>MAGKLGKFQMLGFQHWKGLTSDNHLGAIFQQAPQKATNLMVQLLAFYRGKSLDTFLNSFPTREFEDDNEYYWDVIGSSRRNIPLVEARDENGVVVAANAANVGVGTSPFYLVFPEDWFADGEVIVGNLNQVYPFRILGDARMEGTNAVYKVELMGGNTQGVPAERLQQGERFSIEFAPVEKELSRKVGDVRFTSPVSMRNEWTTIRIQHKVAGNKLNKKLAMGIPMVRNLESGKQVKDTANMWMHYVDWEVELQFDEYKNNAMAWGTSNRNLNGEYMNFGKSGNAIKTGAGIFEQTEVANTMYYNTFSLKLLEDALYELSASKLAMDDRLFVIKTGERGAIQFHKEVLKTVSGWTTFVLDNNSTRVVEKVQSRLHSNALSAGFQFVEYKAPNGVRVRLDVDPFYDDPVRNKILHPMGGVAFSYRYDIWYIGTMDQPNIFKCKIKGDNEYRGYQWGIRNPFTGQKGNPYMSFDEDSAVIHRMATLGVCVLDPTRTMSLIPAILQG[30x];>[25x]MVISINQVRQLYVAKALKANTAALTTAGDIVPKADTAKTTLYFQSMSPAGIVASDKINLKHVLYAKATPSEALAHKLVRYSVTLDADVSATPVAGQNYILRLAFRQYIGLSEEDQYFKYGEVIARSGMTASDFYKKMAISLAKNLENKTESTPLVNIYLISAAAASTDVPVTSATKESDLTATDYNQIIIEETEQPWVLGMMPQAFIPFTPQFLTITVDGEDRLWGVATVVTPTKTVPDGHLIADLEYFCMGARGDIYRGMGYPNIIKTTYLVDPGAVYDVLDIHYFYTGSNESVQKSEKTITLVAVDDGSHTAMNALIGAINTASGLTIATL;>MAGQQGIYCAPDNIVPNRDRVDVGCAPDGAMQLWVMEYEVTGIGKGCAMCKAINPQQAEMLLKSNGIYNGSSYLYKVTRIEQVIVPPCNGLMAEQVVTYKDVVS[10x];>MKTLRTLKISPNAPDINSVWLYKGTMKYFNNGEWETIGGESEPYVLPAATTSTIGGVKKATNVGNLATGAELATVVTKVNAILSALKVADIMVEDAN[15x];>[12x]MADFLNFPRQMLPFSKKTKQWRKDCLLWANQKTFFNYSLVRKSVIHKKINYDLLNGRLHMSDLELVLNPDGIKAAYIPDRLQHYPIMNSKLNVLRGEESKRVFDFKVVVTNPNAISEIEDNKKNELLQRLQEMITDTSISEDEYNIKLEKLNDYYTYEWQDIREVRANELLNHYIKEYDIPLIFNNGFMDAMTCGEEIYQCDIVGGEPVIERVNPLKIRIFKSGYSNKVEDADMIILEDYWSPGRVIDTYYDVLSPKDIKYIETMPDYIGQGAVDQMDNIDERYGFVNQNMIGDEITVRDGTYFFDPANLFTEGIANSLLPYDLAGNLRVLRLYWKSKRKILKVKSYDPETGEEEWNFYPENYVVNKEAGEEVQSFWVNEAWEGTMIGNEIFVNMRPRLIQYNRLNNPSRCHFGIVGSIYNLNDSRPFSLVDMMKPYNYLYDAIHDRLNKAIASNWGSILELDLSKVPKGWDVGKWMYYARVNHIAVIDSFKEGTIGASTGKLAGALNNAGKGMIETNIGNYIQQQINLLEFIKMEMADVAGISKQREGQISQRETVGGVERATLQSSHITEWLFTIHDDVKKRALECFLETAKVALKGRNKKFQYILSDTSTRVMEIDGDEFAEADYGLVVDNSNGTQELQQKLDTLAQAALQTQTLSFSTITKLYTSSSLAEKQRLIEKDEKQIRERQAQAQKEQLEAQQQIAAMQQQQKEAELLQKEEANIRDNQTKIIIAQIQSEGGPDEEDGIMIDDYSPEAKANLAEKIREFDEKLKLDKDKLKLDKKKAETDASIKRQALRKKSSTTNK;>[12x]MVNNINWVKLPVILDRLLRHPLLTDLNLETAIQYTLDFISAMGLPNVYVDKIETIDIKEYRGELPCDLISINQVRLHKNGIALRAMTDNFNAYPTHDHKEGDWYERGEPSFKTQGRVIFTSIKHEKVDISYKAIMLDDEGLPLIPDNPIFLKTLELYIKKEWFTILFDMGKISPAVLNNTQQEYAFKAGQCNNEFVIPSVSEMEAITNMWNQLIPRVTEFRRGFKNLGDKEYIRVH;>[12x]MTYNELIYMVLDELKLSSDDSYYTPDHVIFLLVKYRSFLLKQRYSDIKKQIPDSDYQSICLDLIEVPAISGEPCEGSSYLRSKNKVPTTMMIGNPRVYPMDFYQGEITYISRDRMRYVGYNKFLRNIIYCSKAPDGYLYFKSWNPQFLHLEKVSFNAIFEDAKEASEMACPEENGTICKLEDKEFPIEDALVPPLIELVVKELRGPEYSPKDEDNNAKDDLPDAR;>MAKKKIKRRGKMPPNIFDTGGQSWGQQSSGQFSNAFKGENLGNSIGSIGGAVGGIAQAGISNAQIADTSGIEAQNKAQKNMVVGASSNDDLMSEWGSWNKVKDDYSWKDVRGGSTGQRVTNTIGAAGQGAAAGASVGGPIGAIVGGVVGLGSAIGGWLGGNRKAKRKAKKLNKEAKEANERALTSFETRADNIDTQNDFNMLANFSAYGGPLEFGSGAIGYEFDNRYLNNQEMSAVAKQRLTSLPNSFQALPEMNTYNAFAEGGGLSREKNYGSKKKPYPSVPSGDFAGPHRSYPIPTKADARDALRLAGLHGNESVRRKVLAKYPSLKAFGGSLFDSVVGNNFNQSFTQGIQGMFQQEPEQTVQAANIAKDGGDIKIKEKNKGKFTAYCGGKVTEACIRKGKNSSNPTTRKRATFAQNARNWNAFGGWLNTQGGDFTNGVTFINEGGSHEENPYQGIQIGVDPEGAPNLVEQGEVVYDDYVFSDRMEIPDDIRKEYKLRGKTFAKAAKSAQRESEERPNDPLSTKGLQAAMERIATAQEEARQRKEAHREGNEYPSMFAYGGDTNPYGLALEDPMSVEELEALMVQSGETGEIAPEGNNGNRQTWTRYAPIIGSGLASLSDLFSKPDYDSADLISGVDLGAEAVGYAPIGNYLSYRPLDRDFYINKMNQQAAATRRGLMNTSGGNRLNAQAGILAADYNYGQNMGNLARQAEEYNQQLRERVEAFNRGTNMFNTETGLKASMFNAESRNAAKRARLGQATTVAQLRQGIKDQDAARRSANITNFLQGLGDMGWENEQANWLDTLAKSGVLKMNTKGEYTGGTKKAKGGKVRTKKKKGLTYG[24x]

Virus ΦcrAss001 (Kehishuvirus primarius) was the first representative of this order to be isolated in pure culture from human faecal samples. Here, we present the characterization of ΦcrAss001 using cryo-electron microscopy (cryo-EM), enabling de novo structure building and elucidation of functions for around 1,440 protein subunits constituting the virion, leading to the identification of a novel ‘crass fold’ in the distal part of the tail. The virion possesses a short non-contractile tail extending approximately 44 nm from an icosahedral capsid. The extended tail barrel formed by widely conserved paralogous ring proteins has a high capacity for storage of cargo proteins alongside the capsid cargo zone, ensuring that the proteins required for the initial stages of crassvirus infection are carried inside virions and delivered to the host cell.

One vertex of the capsid contains the dodecameric oligomer of portal protein gp20. The portal is surrounded by the five-fold symmetric capsid vertex, contacting 10 major capsid protein subunits. The 12-fold symmetrical portal oligomer sits within the 5-fold symmetrical capsid vertex. The localized asymmetric reconstruction of the portal–capsid vertex (obtained without imposing symmetry), determined at 3.60 Å resolution, showed that a loop at the peripheral area of the wing domain, residues 268–319, is flexible and can adopt two preferred conformations (types A and B) in interacting with the C5-symmetric capsid vertex. In the type A conformation, residues 277–290 of this ‘capsid-adaptable loop’ are oriented radially away from the portal’s tunnel axis, whereas in the type B conformation residues 292–306 of the loop are arranged tangentially to the portal’s circumference. In 2 of the 12 subunits of the portal protein, these loops were not resolved in either conformation (denoted ‘x’), resulting in the A-B-x-A-B-A-B-A-x-B-A-B order of the conformational states, counting clockwise if viewed from outside of the capsid. The result is a pseudo-five-fold symmetrical arrangement of capsid-adaptable loops around the 12-subunit oligomer, assisting the formation of optimal interactions with the five-fold symmetric capsid vertex. The portal oligomer positioned in the vertex occludes the binding site of the capsid auxiliary protein gp36, which is substituted by two copies of the portal vertex specific auxiliary protein, gp57. The gp57 dimer has approximate two-fold symmetry, reinforced by disulfide bonds between residues 47–47 and 25–88 of the two subunits. Notably, hexameric capsomers bordering the unique vertex contain trimer capsid fibres of gp21, in contrast to the hexamers bordering other pentameric vertices, which contain dimeric capsid fibres of gp29.>MSEHREGTLFYDTETGRYDIRFDLESFYGGLHCGECFDVKVKDVWVPVRIEMGDDWYLVGLNV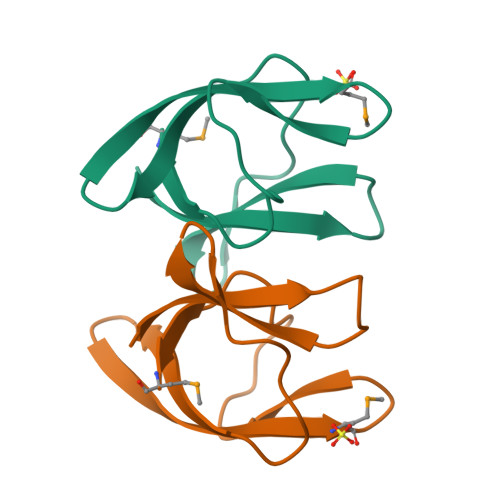SRLDGLRVRMLEHHHHHH[2x]>[4x]GAMGS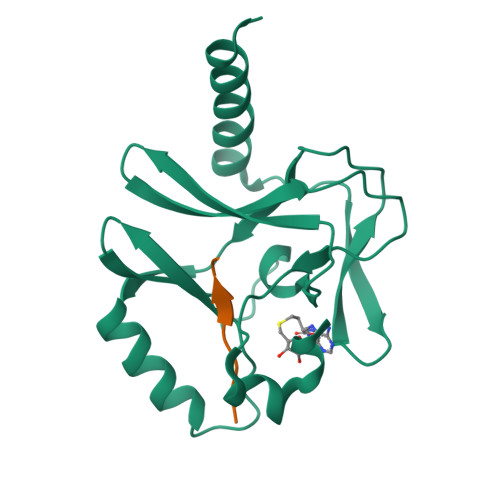RKSKAELQSEERKRIDELIESGKEEGMKIDLIDGKGRGVIATKQFSRGDFVVEYHGDLIEITDAKKREALYAQDPSTGCYMYYFQYLSKTYCVDATRETNRLGRLINHSKCGNCQTKLHDIDGVPHLILIASRDIAAGEELLFDYGDRSKASIEAHPWLKH;>AKRHRKVLRD[4x]>[2x]HTIFSSLEVNGVNQGLGEGVRVPTYNGPIEDVTSASIACNGSPNTVASTSKVITVQAGTNVTAIWRYMLSTTGDSPADVMDSSHKGPTIAYLKKVDNAATASGVGNGWFKIQQDGMDSSGVWGTERVINGKGRHSIKIPECIAPGQYLLRAEMIALHAASNYPGAQFYMECAQLNVVGGTGAKTPSTVSFPGAYSGSDPGVKISIYWPPVTSYTVPGPSVFTC

Lytic polysaccharide monooxygenases (LPMOs; also designated PMOs) are copper metalloenzymes that perform unique redox chemistry resulting in disruption of polysaccharide chains by oxygen atom insertion at the glycosidic bond. The LPMO active site is highly conserved and contains a mononuclear Cu2+ center within a “histidine brace” motif in which the copper is coordinated by the N-terminal histidine amino group, the Nδ atom of His1 and the Nε atom of a second conserved histidine in the equatorial plane. In the Cu2+ resting state, the remaining equatorial and axial positions are each occupied by a water molecule. Of particular commercial and biotechnological interest is the ability of fungal LPMOs to catalyze the oxidative cleavage of recalcitrant crystalline cellulose at the C1 and/or C4 position, thereby enhancing polysaccharide depolymerization by increasing glucan access to hydrolytic enzymes and ensuring efficient bioconversion.

LPMOs are expected to catalyze oxygen insertion under acidic conditions since they function synergistically alongside cellulases which show optimum activity at pH 3.5–5.5.65–67 Given the surprising role of a neutral His157 as a proton donor to the activated dioxygen species in our structure, we sought to probe the protonation state of His157 when exposed to acidic buffer conditions. To further support our acidic pH structure obtained by vapor exchange, a 1.5 Å X-ray dataset was collected on a crystal directly soaked in acidic buffer. Furthermore, the neutron and X-ray crystal structures of the resting state NcLPMO9D at low pH show that His157 remains singly protonated when exposed to acidic conditions. The position of His157 at pH 4.4 superimposes to its position at pH 6.0. In this position, Nδ-protonation would sterically clash with the backbone amide proton, further supporting the single Nε-protonation state observed in our neutron structure (Fig. S6 and S7†) which coincides with unrestrained refinement studies of the protonation state of second-shell His residues. The barricaded active site observed in crystallo and electropositive environment of the copper potentially play a role in maintaining the observed single histidine protonation state and prevent formation of protonation pathways to the active site. However, the single protonation of His157 solely at the Nε position in our crystal structures does not rule out formation of the doubly protonated second shell histidine residue under similar acidic operando conditions where the active site would not be barricaded by crystal packing.A 1.5-MDa RTX adhesin [MpAFP (Marinomonas primoryensis antifreeze protein)] with ice-binding activity was found on the surface of the Gram-negative bacterium, Marinomonas primoryensis, from Antarctica. MpAFP can be divided into five distinct Regions (RI–RV) that include the highly repetitive RII (Region II) and the moderately repetitive RIV (Region IV). RII consists of approximately 120 tandem copies of a perfect 104-aa repeat that account for over 90% of the mass of the 1.5-MDa protein. We hypothesized that MpAFP_RII serves as a Ca2+-dependent extender domain to project the ice-binding RIV away from other cell surface molecules in order to bind M. primoryensis to ice.

The crystal structure of the RII tetra-tandemer from MpAFP was solved to a resolution of 1.8 Å by the molecular replacement method using the RII-tandemer (PDB: 4 KDV) as the search model. The RII tetra-tandemer is roughly 190 Å long and 23×28 Å in cross-section. There are 104 Ca2+ ions bound to the four RII tetra-tandemers within the unit cell of the crystal, with a minimum of 24 Ca2+ binding to each tetra-tandemer binding. Each individual 104-aa repeat of the RII tetra-tandemer folds as a Ca2+-dependent Ig-like β-sandwich that contains seven antiparallel and two short parallel β-strands, and two short α-helices. Seven β-strands (β1–β6 and β9) and the two α-helices (α1 and 2) help form the compact core region of the Ig-like domain, whereas β7 and β8 comprise a β-hairpin that protrudes from the core, and points toward the N-terminal end of the structure. The four tandem Ig-like β-sandwiches of the RII tetra-tandemer are aligned in a highly extended fashion. Each repeat is rotated by approximately 90° relative to its neighbour(s), forming an internal 4-fold symmetry within the RII tetra-tandemer. Ca2+ ions are also coordinated at the linker regions between the neighbouring repeats. Thus the inter-repeat Ca2+ mediates the interaction between the tandem RII domains by keeping the C-terminal end of one repeat in close proximity to the β-hairpin (β7 and 8) from the subsequent repeat. Furthermore, evaluation of the atomic structure with the solution scattering data using CRYSOL also yields a good fit, corroborating that the crystal structure is representative of the structure of the protein in solution.

>[4x]MASSHHHHHHSSGLVPRGSHMTEATAGTVTVNAITSDDVINASEAAGTVAVSGTATGGDIAEGDTVTLEINGETYTTTVDANGEWSVDVAGSDLAADTAFDAVVTSSDAAGNTVDTTGSSTHTVDTEATAGTVTVNAITSDDVINASEAAGTVAVSGTATGGDIAEGDTVTLEINGETYTTTVDANGEWSVDVAGSDLAADTAFDAVVTSSDAAGNTVDTTGSSTHTVDTEATAGTVTVNAITSDDVINASEAAGTVAVSGTATGGDIAEGDTVTLEINGETYTTTVDANGEWSVDVAGSDLAADTAFDAVVTSSDAAGNTVDTTGSSTHTVDTEATAGTVTVNAITSDDVINASEAAGTVAVSGTATGGDIAEGDTVTLEINGETYTTTVDANGEWSVDVAGSDLAADTAFDAVVTSSDAAGNTVDTTGSSTHTVD> GGGGG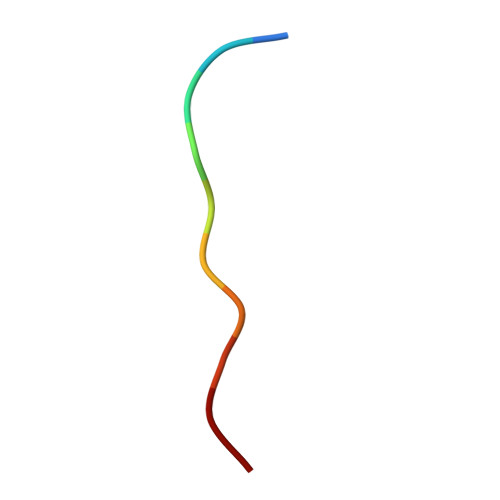GGGGG> AATTVNGGTVHFKGEVVNAACAVDAGSVDQTVQLGQVRTASLAQEGATSSAVGFNIQLNDCDTNVASKAAVAFLGTAIDAGHTNVLALQSSAAGSATNVGVQILDRTGAALTLDGATFSSETTLNNGTNTIPFQARYFAT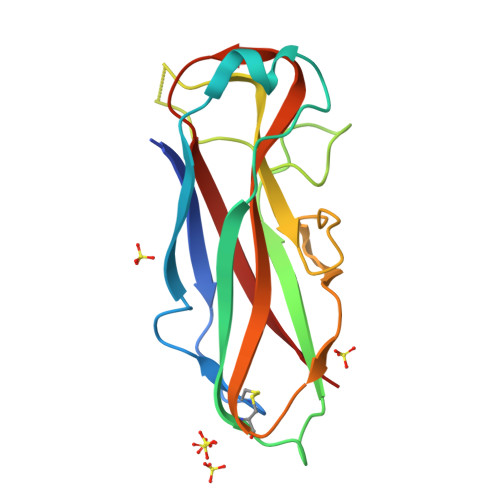GAATPGAANADATFKVQYQ>MTVVSAFLVPGTPLPQLKPEVPSWGQLAAATERAGKALAASRPDVVLVYSTQWLAVLDQQWLTRPRSEG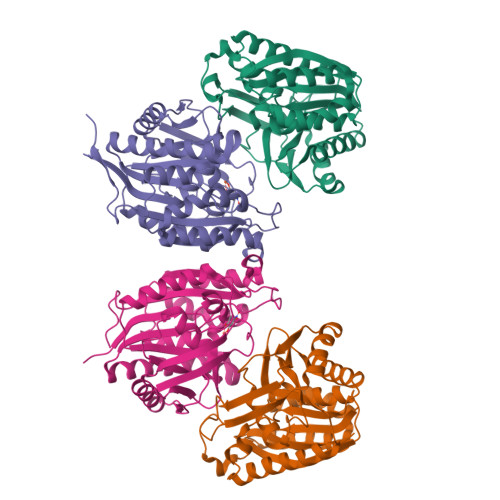VHVDENWYEFGDLAYDIRADTALAEACVTSSPLHGVHARGVNYDGFPIDTGTITACTLMGIGTDAFPLVVGSNNLYHSGEITEKLAALAVDCAKDQNKRVAVVGVGGLSGSLFREEIDPREDRIANEEDDKWNRRVLKLIEAGDVSALREAMPVYAKEARVDMGFKHLHWILGALKGKFSGANVLGYGPSYGSGAAVIEFRL[2x];>[2x]MQGEIIAGFLAPHPPHLVYGENPPQNEPRSQGGWEVLRWAYERARERLDAMKPDVLLVHSPHWITSVGHHFLGVPELSGKSVDPIFPNVFRYDFSLNVDVELAEACAEEGRKAGLVTKMMRNPKFRVDYGTITTLHLIRPQWDIPVVGISANNSPYYLNTKEGMSEMDVLGKATREAIRKTGRKAVLLASNTLSHWHFHEEPTIPEDMSKEYPATMAGYQWDIRMIELMRQGKTSEVFKLLPQFIDEAFAEVKSGAFTWMHAAMQYPELAAELFGYGTVIGTGNAVMEWDLRKAGLSMLGAADQKQRSAAVA> ACTKNAIAQTGFNKDKYFNGDVWYVTDYLNLEPDDVPKRYCAALAAGTASGKLKEALYHYDPKTQDTFYDVSELQVESLGKYTANFKKVDKNGNVKVAVTAGNYYTFTVMYADDSSALIHTCLHKGNKDLGDLYAVLNRNKDAAAGDKVKSAVSAATLEFSKFISTKENNCAYDNDSLKSLLTK

Another heme b containing protein class with a novel type of nitrite reaction is the nitrophorins (NPs) that originate from the saliva of the blood feeding insect Rhodnius prolixus. At least five isoforms appear concurrently in the insect saliva, termed NP1–4 and NP7.13,14 The biological function of the ferriheme b NPs has been established as an NO transporter. Interestingly, NPs were found to be able to convert nitrite into NO via a ‘nitrite-only’ mechanism with the stoichiometry of the nitrite disproportionation reaction. In summary, the key factors that facilitate the nitrite dismutase reaction of NPs have been established to be the heme ruffling and an extended H-bonding network at the active site which helps to keep the proximal His residue neutral.

In a previous study, we showed that the NP4(D30N) variant has almost no nitrite dismutase activity, thus concluding that Asp30 is a key residue for its activity. Inspired by this result, we measured the EPR spectrum of the nitrite complex with NP4(D30N). Interestingly, it shows a significantly increased ratio of HALS species (≈60%) compared to that of the wt NP4[NO2–] (Table S1†). It shows that nitrite binds to the heme iron in an N-bound nitro form like in the cases of NP4[NO2–] and NP4(L130R)[NO2–]. The two mutations D30N and L130R, however, dramatically interfere with the distal heme pocket in the sense that the Asp30···water···water···nitrite H-bonding network of the wt protein is disrupted in both cases (Fig. S6†). In the cases of the nitrite complexes of NP4(L130R) and NP4(D30N), a negatively charged proximal histidinate—resulting from the perturbation of the H-bonding network in the distal heme pocket—would lead to a weakened Fe–Nnitrite coordination compared to that of the wt protein due to the trans effect or electron–electron (anion–anion) repulsion. In line with this are the slightly larger Fe–Nnitrite bond distances observed in the complexes of NP4(L130R)[NO2–] (2.1 Å) and NP4(D30N)[NO2–] (2.1 Å) compared to that of NP4[NO2–] (2.0 Å) (compare Fig. 3). Similarly, NP4(D30N) was reported to have a lower redox potential than that of the wt NP4 (–429 mV for NP4(D30N) vs. –384 mV for wt NP4 at pH 5.0),70 however, it cannot react with nitrite, which clearly argues for the role of the H-bonding network of NPs in determining the nitrite dismutase activity.> GAMGSNINEPSGEAADIISQVADSHAIKYYNAADWQAEDNALPSLAELRDLVINQQKRVLVDFSQISDAEGQAEMQAQFRKAYGVGFANQFIVITEHKGE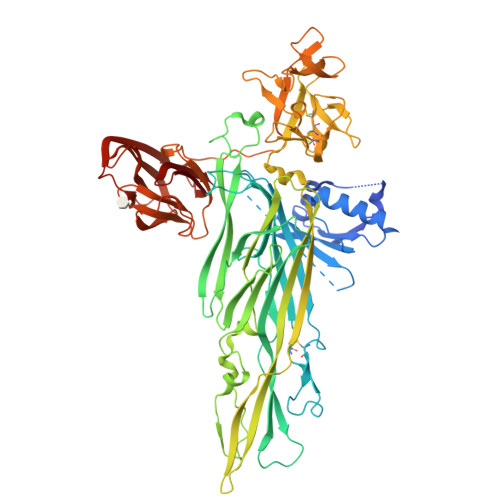LLFTPFDRTEEIDPALLEAPRTAALLGASGFASPAPANSETNTLPHVAFYISVNRAISDEECTFNNSWLWKNEKGSRPFCKDANISLIYRVNLERSLQYGIVGSATPDAKIVRISLDDDSTGAGIHLNDQLGYRQFGASYTTLDAYFREWSTDAIAQDYRFVFNASNNKAQILKTFPVDNINEKFERKEVSGFELGVTGGVEVSGDGPKAKLEARASYTQSRWLTYNTQDYRIERNAKNAQAVSFTWNRQQYATAESLLNRSTDALWVNTYPVDVNRISPLSYASFVPKMDVIYKASATETGSTDFIIDSSVNIRPIYNGAYKHYYVVGAHQSYHGFEDTPRRRITKSASFTVDWDHPVFTGGRPVNLQLASFNNRCIQVDAQGRLTANMCDSQQSAQSFIYDQLGRYVSASNTKLCLDGAALDALQPCNQNLTQRWEWRKGTDELTNVYSGESLGHDKQTGELGLYASSNDAVSLRTITAYTDVFNAQESSPILGYTQGKMNQQRVGQDNRLYVRAGAAIDALGSASDLLVGGNGGSLSSVDLSGVKSITATSGDFQYGGQQLVALTFTYQDGRQQTVGSKAYVTNAHEDRFDLPDAAKITQLKIWADDWLVKGVQFDLN> AEQAQPKTPENSSTEQPTVKATQTTEQAITEKQQQVTEKQAIVDQKQQVADTAKKEKDAIDQSVKDQQAVVDQNKDALDQSQQAVTDQQAVVDEAKKVVDEATPSAIEKAKEQVATDTQAVDEQQKVVDQAQTDVNQQQAVVDEKAKETNAAKVQNEKDQQAVTAAKQEQAKLEELAKNAEAEKVKAEKEQAAKEAELANKQKEEAKAKDQKTKDDQAVADQQTVVTTSQEKVTDAKADTAAKQADLTAKENALKDKQAATKQAQNTLDNSKEELKGHKGINLPPKFSADYDTKLSAEEIATLEKTALEMNKNFPTSKEDEKNKDVMWDIQHLSADQKKELS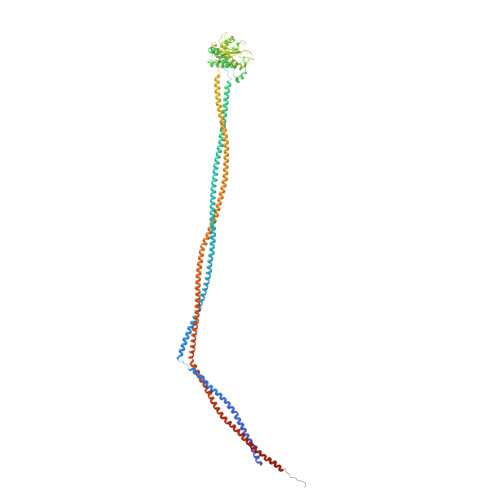VYTTELLNDVRKKLGLSQLSVSDQSIKFAWDIAKYSDTGEYMHDVIAINKAAKENGFKEYPGMNYYENLGGGYYETENGKVSKYTLQESIRKMLVNMLFDDGRLGYSHLHSLLQDGKTALGVSLSGEKNSISPKIHIISYGKEKLEDSSQYQNGEVASMKSKEELQQEIASNQEKLATAQQAESDAQQARSASQQALNTAKTTQATAEKELSVHKATLANLQAVATKSTTNYEEKVRQTATAEKSLQQTKDQLATINELIQNRAAVLEKAKTNVAEAQAIEQTSAKVLKEKQEAQKAEENTLNSLKEVLDLAKENLNQKQVALKTSTRSLSRLENAQPTYEKALNELNKAEAAVVQAQEAYENSMKSLEELKEQQAVATLAYAQAQEDLSNAKLELQQYQGVLRDLEAQQAEQRRQEALQEQVAKEQQRLEREAKQNQTLVASAT>[8x]GUUUAUAGACAUAGCCUUGUGUAUGACUGUCUAAUCAACAGUGCAAGGAAUUAGUUGUGCUCUCAAAAGGAGUUAUGUGAAGGAAAGAUUAAAUGGAUACAUUUAAUUAAGUACAAUUACUACAAAAUCUAUAAUGACUGGGUAAGUCACCCGUAAGAAGGAUGAGUUAGUAGAGAUAUAAUAAUAUCUUACAGUUCAACUGAUGUGCAAGUUUAUAAGUAGACGUAGUGUGAAAGACUUAUCGCUAACGCAAUAGACGUUAUCUCGAAAGGAUAAAAGAAACCAAGAAGAUAUACAAAUUGGUAACUUGUAUAAGCCCUUGGUAAUACCAAAUAAGUUAGUUCCUCAUGAUGUCGUGGAAACAUGACUAUAAGAUAAGUUGAAUUCGAUAGUAGCCCAAGAGGAAUCNNNNNNNNNNNNNNNNNNNNNNNNNNNNNNNNNNNNNNNNNNNNNNNNNNNXGAUUGUGCCUUGAAAAAGGUGGGUGAGGUCUGUGGGUAAAAAUUAAUUCCCAUCUGGUUUUGGAUUUUCUUCGGAAAAUUGGUGCAAGAAGCGUGGAGUUGCUAACCAUUGCUCAGACUUGUAUCGCCAGUAGCACGAUAACGAUAUUUAUGAAUGUUGUAAGGUGAAUAAAAGCCUAUGAUUUGUGAAC

Here we report three-dimensional structures of three large ornate bacterial RNAs using cryo-electron microscopy (cryo-EM). GOLLD (Giant, Ornate, Lake- and Lactobacillales-Derived), ROOL (Rumen-Originating, Ornate, Large) and OLE (Ornate Large Extremophilic) RNAs form homo-oligomeric complexes whose stoichiometries are retained at lower concentrations than measured in cells. Unexpectedly, the three structures are stabilized not by proteins but by other copies of the same RNA molecule in ornate quaternary assemblies with many intermolecular bridges, a phenomenon that has not previously been observed for natural RNA molecules. Extensive intramolecular and intermolecular A-minor interactions, kissing loops, an unusual A–A helix and other interactions stabilize the three complexes.

ROOL is a class of RNAs that is encoded in a wide variety of bacterial prophages and phages, often near tRNA islands. The 659-nt ROOL env-120, discovered in cow rumen, produces visually clear, symmetric particles in cryo-EM micrographs. The 3.1 Å reconstructed map reveals a closed, hollow nanocage structure that comprises 8 chains with dihedral symmetry and a diameter of approximately 280 Å, larger than the maximal dimension of a bacterial ribosome (approximately 250 Å). Each chain has a secondary structure that is consistent with the stems P1 to P19 proposed previously by covariation analysis, including the pseudoknot P10. The ROOL quaternary complex is an octameric nanocage, with a top and bottom half-shells, each formed by 4 chains, hereafter labelled chains 1–4 and 1′−4′. Within a half-shell, each chain forms 8 bridges with its neighbours, 4 on each side, labelled B1–B4. An A-minor interaction (B2) and a novel quaternary kissing loop (B1) further glue together the chains in the half-shell. The P7 stem is not always conserved, but a second circle of RNA, involving a quaternary kissing loop (B4), is highly conserved in evolution, and was identified as tertiary interaction by previous covariation analysis. As opposed to a simple dimer such as the OLE interface, where each chain interacts with a single partner, in the ROOL complex, each chain reaches over and interacts with two chains in the other half-shell. These interactions favour the full cage assembly, as opposed to isolated dimers.>MSSSHSRAGQSAAGAAPGGGVDTRDAEMPATEKDLAEDAPWKKIQQNTFTRWCNEHLKCVSKRIANLQTDLSDGLRLIALLEVLSQKKMHRKHNQRPTFRQMQLENVSVALEFLDRESIKLVSIDSKAIVDGNLKLILGLIWTLILHYSISMPMWDEEEDEEAKKQTPKQRLLGWIQNKLPQLPI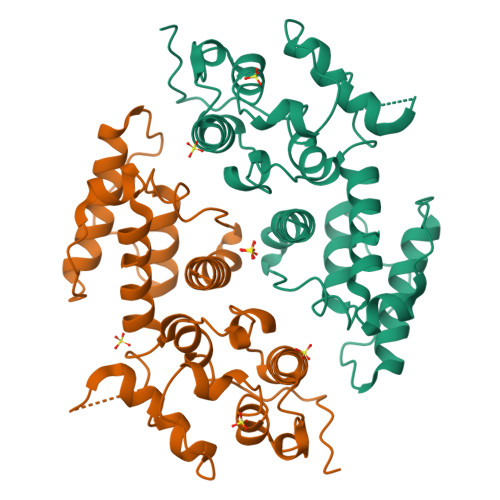TNFSRDWQSGRALGALVDSCAPGLCPDWDSWDASKPVTNAREAMQQADDWLGIPQVITPEEIVDPNVDEHSVMTYLSQFPKAKLKPGAPLRPK[2x]The Na+/Ca2+ exchanger (NCX), belonging to the CaCA (Ca2+/Cation antiporter) superfamily of secondary active transporters, forms one of major pathways to mediate Ca2+ fluxes across the cell membrane and significantly contributes to the regulation of Ca2+-dependent events in various cell types. The NCX is a bi-directional and reversible transporter, and utilizes the electrochemical gradient of Na+ to exchange 3 Na+ ions for 1 Ca2+ across the membrane, thus performing electrogenic transport. The f-loop consists of two tandem calcium-binding domains (CBD1 and CBD2), which exert allosteric regulation of NCX activity by binding cytosolic Ca2+. In addition to the CBD1/2, the exchanger inhibitory peptide (XIP) region located within the f-loop has also been determined to block NCX activity in response to high concentration of cytosolic sodium ion ([Na+]in).

In this work, we purified the recombinant human full-length wild-type (WT) NCX1.3 and determined its complex structure bound with SEA0400 by using the cryo-electron microscopy (cryo-EM) method. The final selected particles were subjected to 3D refinement and yielded an EM map of 3.5-Å resolution, which includes many well-resolved features and clear densities of main-chains, side-chains. NCX1.3 structure consists of 10 transmembrane helices (TMs 1–10) and the large intracellular regulatory domains CBD1 and CBD2, with both N- and C-termini located at the extracellular side. The conserved residues for coordinating Na+ or Ca2+ are accessible from the intracellular side, indicating that the current NCX1.3 structure is trapped in an inward-facing conformation, which is stabilized by both the XIP region and SEA0400 antagonist. Structural comparison between NCX1.3IF and mjNCXOF also reveals a steric hinderance between the XIP region of NCX1.3 and TMs1/6 helices of mjNCXOF, suggesting that the XIP region in its current position would prohibit conformational transition from the inward-facing to outward-facing state. It inserts into a juxtamembrane, highly negatively charged groove formed by TM1, β2, TM2, TM7, TM8, H1, and CBD2, and is largely stabilized by complementary electrostatic interactions. The SEA0400 molecule is allocated within a negatively charged cavity surrounded by TM2ab, TM4, TM5, and TM8. In fact, the pocket and passageway are separated by the TM2ab helix, indicating that SEA0400 inhibits transport activity through an allosteric fashion. The ethoxyaniline group of SEA0400 forms hydrogen bonding interaction with T138TM2ab and hydrophobic interactions with F248TM5. In agreement, since SEA0400 stabilizes the straight α-helical conformation and disrupts the local backbone dynamics of TM2ab, the association of SEA0400 allosterically inhibits the conformational transition.

> MYNMRRLSLSPTFSMGFHLLVTVSLLFSHVDHVIAETEMEGEGNETGECTGSYYCKKGVILPIWEPQDPSFGDKIARATVYFVAMVYMFLGVSIIADRFMSSIEVITSQEKEITIKKPNGETTKTTVRIWNETVSNLTLMALGSSAPEILLSVIEVCGHNFTAGDLGPSTIVGSAAFNMFIIIALCVYVVPDGETRKIKHLRVFFVTAAWSIFAYTWLYIILSVISPGVVEVWEGLLTFFFFPICVVFAWVADRRLLFYKYVYKRYRAGKQRGMIIEHEGDRPSSKTEIEMDGKVVNSHVENFLDGALVLEVDERDQDDEEARREMARILKELKQKHPDKEIEQLIELANYQVLSQQQKSRAFYRIQATRLMTGAGNILKRHAADQARKAVSMHEVNTEVTENDPVSKIFFEQGTYQCLENCGTVALTIIRRGGDLTNTVFVDFRTEDGTANAGSDYEFTEGTVVFKPGDTQKEIRVGIIDDDIFEEDENFLVHLSNVKVSSEASEDGILEANHVSTLACLGSPSTATVTIFDDDHAGIFTFEEPVTHVSESIGIMEVKVLRTSGARGNVIVPYKTIEGTARGGGEDFEDTCGELEFQNDEIVKIITIRIFDREEYEKECSFSLVLEEPKWIRRGMKGGFTITDEYDDKQPLTSKEEEERRIAEMGRPILGEHTKLEVIIEESYEFKSTVDKLIKKTNLALVVGTNSWREQFIEAITVSAGEDDDDDECGEEKLPSCFDYVMHFLTVFWKVLFAFVPPTEYWNGWACFIVSILMIGLLTAFIGDLASHFGCTIGLKDSVTAVVFVALGTSVPDTFASKVAATQDQYADASIGNVTGSNAVNVFLGIGVAWSIAAIYHAANGEQFKVSPGTLAFSVTLFTIFAFINVGVLLYRRRPEIGGELGGPRTAKLLTSCLFVLLWLLYIFFSSLEAYCHIKGF N-((2R,4S)-2-butyl-4-(3-(2-fluorophenyl)ureido)-5-methyl-3-oxohexyl)-N-hydroxyformamide 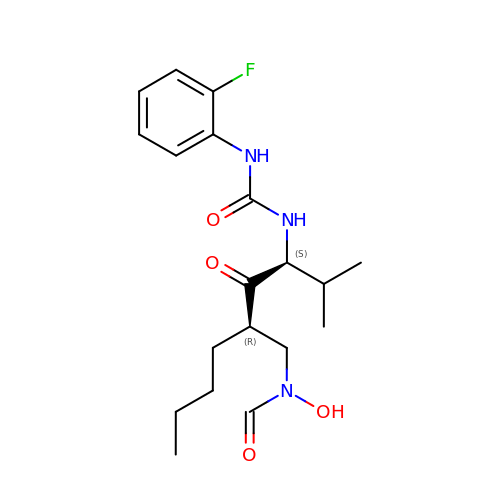| C19 H28 F N3 O4 | OWFALUNDSZEADU-PBHICJAKSA-N>GSHHKAVLAVRREDVNAWERRAPLAPKHIKGITNLGYKVLIQPSNRRAIHDKDYVKAGGILQEDISEACLILGVKRPPAAALMSRKTYAFFSHTIKAQEANMGLLDEILKQEIRLIDYEKMVDHRGVRVVAFGQWAGVAGMINILHGMGLRLLALGHHTPFMHIGMAHNYRNSSQAVQAVRDAGYEISLGLMPKSIGPLTFVFTGTGNVSKGAQAIFNELPCEYVEPHELKEVSQTGDLRKVYGTVLSRHHHLVRKTDAVYDPAEYDKHPERYISRFNTDIAPYTTCLINGIYWAANTPRLLTRQDAQSLLAPGKFSPAGVEGCPALPHKLVAI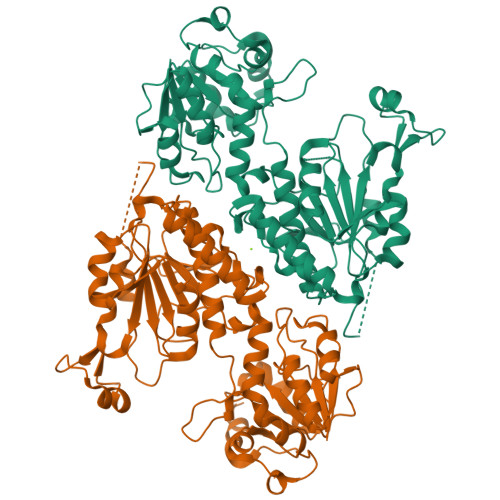CDISADTGGSIEFMTECTTIEHPFCMYDADQHIIHDSVEGSGILMCSIDNLPAQLPIEATECFGDMLYPYVEEMILSDATQPLESQNFSPVVRDAVITSNGTLPDKYKYIQTLRESRE[4x]>[4x]GSMELLQGKTFVVMGVANQRSIAWGI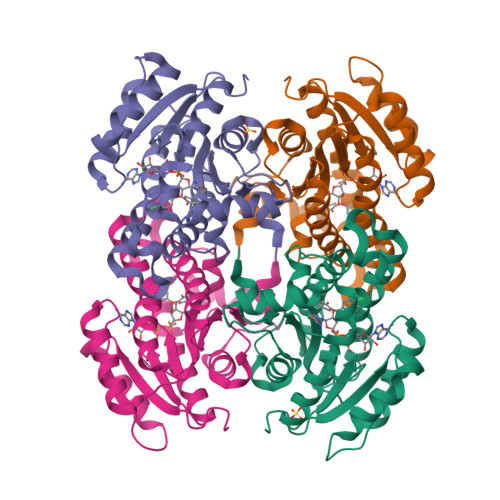ARSLHNAGAKLIFTYAGERLERNVRELADTLEGQESLVLPCDVTNDEELTACFETIKQEVGTIHGVAHCIAFANRDDLKGEFVDTSRDGFLLAQNISAFSLTAVAREAKKVMTEGGNILTLTYLGGERVVKNYNVMGVAKASLEASVKYLANDLGQHGIRVNAISAGPIRTLSAKGVGDFNSILREIEERAPLRRTTTQEEVGDTAVFLFSDLARGVTGENIHVDSGYHILG>[2x]MHHHHHHMLENKLGIINQLELNRVEERVSK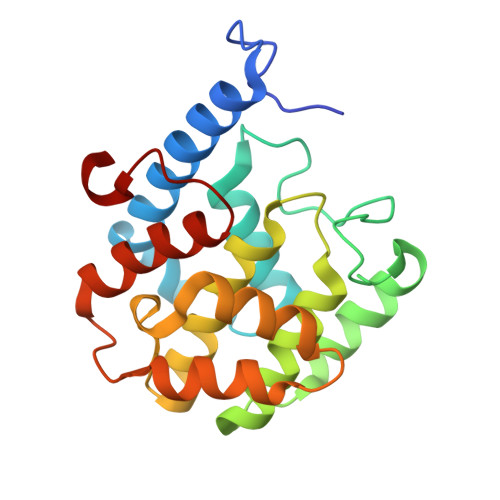ENAKRLYDSGDIDRIEVGTFKGLSYIHNYLFEDIYEFAGKVRSQNISKGNFRFAPVMYLEIALEHIDKMPQRNLDEIVAKYVEMNIAAPFREGNGRATRIWLDLILKKELKRVVDWNLINKEDYLSAMERSPVKDLEIKYLISNALTDKINDREIFMKGIDISYYYEGYTEYNVDEL> MDVDEMLKQVEILRRLG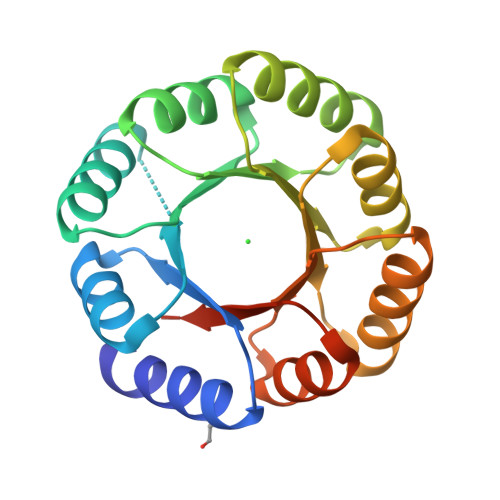AKQIAVRSDDWRILQEALKKGGDILIVDATDVDEMLKQVEILRRLGAKQIAVRSDDWRILQEALKKGGDILIVDATDVDEMLKQVEILRRLGAKQIAVRSDDWRILQEALKKGGDILIVDATDVDEMLKQVEILRRLGAKQIAVRSDDWRILQEALKKGGDILIVDATGLEHHHHHH>[3x]MHADSAPSTTSSQAYAPDARNDAVLVYVNGQFVPRHQAVVSVFDAGYVCGDGVWEGVRLVDGRIVSFDAHIDRMYEGAKSIALDIGMTRAQTKQVVVDTFLRNGMRDGAHARLMVTRGVK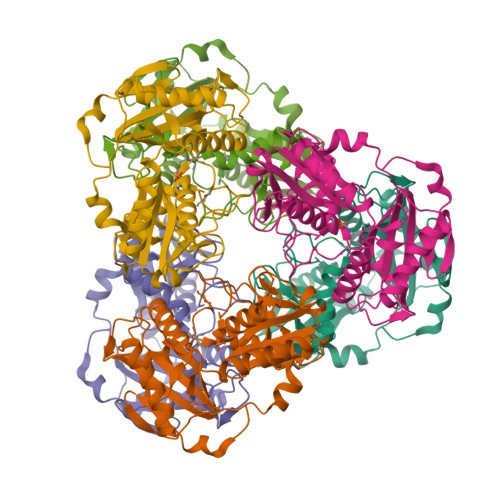KTPNQDPRFIIGGATVVCVAEHKVVTPEAKRNGLKLFTSTLRCSGPDVFDLRLKSHSRLNLIQALIQAIQAGADEALMLDPNGFVSSCNSTNFFAVRNGALWTSSGRYCFNGITRATVVRLAREAGIPVHEGDFTLAEVYAADEAFVTGTLAGLTPVSSVDGRALVPLGPLTQRLDALYRAYIASANEAHGALPAAA> MTESYDVVVVGGGPVGLATAWQVAERGHRVLVLERHTFFNENGGTSGAERHWRLQYTQEDLFRLTLETLPLWRALESRCERRLIHEIGSLWFGDTDVVTNEGQISGTAAMMDKLSVRYEWLKATDIERRFGFRGLPRDYEGFLQPDGGTIDVRGTLAALFTLAQAAGATLRAGETVTELVPDADGVSVTTDRGTYRAGKVVLACGPYTNDL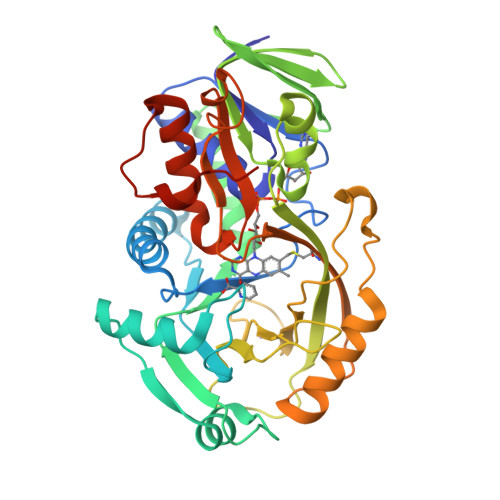LEPLGARLAYSVYEMAIAAYRQATPVTEAPFWFAFQQPTPQDTNLFYGFGHNPWAPGEFVRCGPDFEVDPLDHPSAATGVADRRQMDRLSGWLRDHLPTVDPDPVRTSTCLAVLPTDPERQFFLGTARDLMTHGEKLVVYGAGWAFKFVPLFGRICADLAVEDSTAYDISRLAPQSALLEHHHHHH> ATFGRATHVVVRALPESLAQQALRRTKGDEVDFARAERQHQLYVGVLGSKLGLQVVQLPADESLP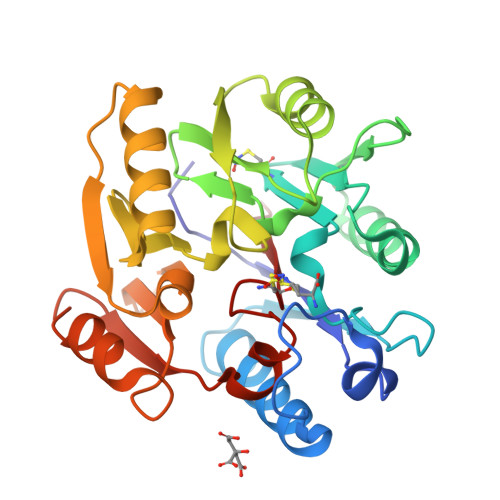DCVFVEDVAVVCEETALITRPGAPSRRKEADMMKEALEKLQLNIVEMKDENATLDGGDVLFTGREFFVGLSKRTNQRGAEILADTFKDYAVSTVPVVDALHLKSFCSMAGPNLIAIGSSESAQKALKIMQQMSDHRYDKLTVPDDTAANCIYLNIPSKGHVLLHRTPEEYPESAKVYEKLKDHMLIPVSNSELEKVDGLLTMSSVLINKK>GMQAPRLRVGIFDDGSSTVNMAEKLDSVGHYVTVLHAPEDIRDFELVVIDAHGVEGYVEKLSAFARRGQMFLHTSLTHGITVMDPLETSGGIVMSAHPIGQDRWVASALDELGETIVGLLVGELGGSIVEIADDKRAQLAAA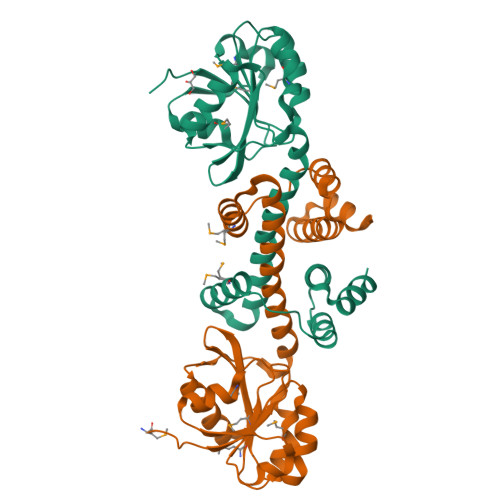LTYAGFLSTLQRDASYFLDEFLGDPDVTSDIVMDSAQQFQALPSLDEVIAQYDSINNPGRQRLFRDLARRQAEISRAQDIELWAIQKEDR[2x]>[2x]SETSRTAFGGRRAVPPNNSNAAEDDLPTVELQGVVPRGVNLQEFLNVTSVHLFKERWDTNKVDHHTDKYENNKLIVRRGQSFYVQIDFSRPYDPRRDLFRVEYVIGRYPQENKGTYIPVPIVSELQSGKWGAKIVMREDRSVRLSIQSSPKCIVGKFRMYVAVWTPYGVLRTSRNPETDTYILFNPWCEDDAVYLDNEKEREEYVLNDIGVIFYG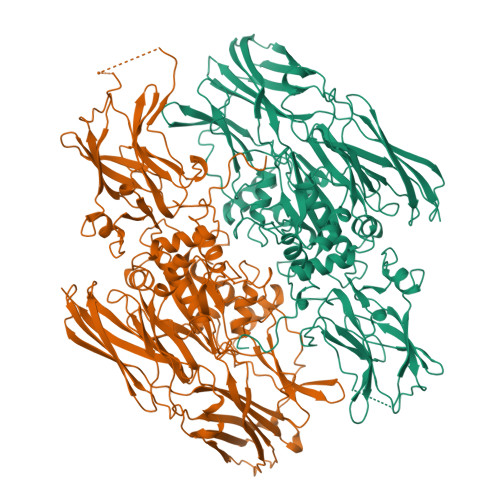EVNDIKTRSWSYGQFEDGILDTCLYVMDRAQMDLSGRGNPIKVSRVGSAMVNAKDDEGVLVGSWDNIYAYGVPPSAWTGSVDILLEYRSSENPVRYGQCWVFAGVFNTFLRCLGIPARIVTNYFSAHDNDANLQMDIFLEEDGNVNSKLTKDSVWNYHCWNEAWMTRPDLPVGFGGWQAVDSTPQENSDGMYRCGPASVQAIKHGHVCFQFDAPFVFAEVNSDLIYITAKKDGTHVVENVDATHIGKLIVTKQIGGDGMMDITDTYKFQEGQEEERLALETALMYGAKKPLNTEGVMKSRSNVDMDFEVENAVLGKDFKLSITFRNNSHNRYTITAYLSANITFYTGVPKAEFKKETFDVTLEPLSFKKEAVLIQAGEYMGQLLEQASLHFFVTARINETRDVLAKQKSTVLTIPEIIIKVRGTQVVGSDMTVTIQFTNPLKETLRNVWVHLDGPGVTRPMKKMFREIRPNSTVQWEEVCRPWVSGHRKLIASMSSDSLRHVYGELDVQIQRRPSM> MAEGNTLISVDYEIFGKVQGVFFRKHTQAEGKKLGLVGWVQNTDRGTVQGQLQGPISKVRHMQEWLETRGSPKSHIDKANFNNEKVILKLDYSDFQIVK

Here we used a pair of thermophilic/mesophilic acylphosphatases homologues (acylphosphatase from hyperthermophilic archaeon Pyrococcus horikoshii (PhAcP) and human common-type acylphosphatase (HuAcP)) as a model to study how local flexibility of the active site affects the enzymatic activity. Despite remarkable conservation of sequence and structure at the active site, the catalytic activity of the thermophilic PhAcP is significantly poorer as compared with its mesophilic homologue HuAcP at low temperatures. The salt-bridge between the active-site residue Arg-20 and the C-terminal carboxyl group is found only in thermophilic PhAcP but not in mesophilic HuAcP. Taken together, our data suggest that the presence of the salt-bridge between the C-terminal carboxyl group and the active-site arginine residue increases the activation energy that results in a stronger temperature dependency of the enzymatic activity.

Importantly, the activation energy (52.5±2.5 kJmol−1) for HuG99 was analogous to that for PhWT (49.1±1.4 kJmol−1), while the activation energy for HuA99 (29.5±1.9 kJmol−1) and HuWT (37.6±3.1 kJmol−1) was comparable to that for PhG91A (32.1±1.7 kJmol−1). To provide further insights into how the active-site salt-bridge affected the enzymatic activity of acylphosphatases, we calculated and summarized the free energy (ΔG#), enthalpy (ΔH#), and entropy (ΔS#) of activation, as well as the changes of these parameters (ΔΔG#, ΔΔH#, ΔΔS#) upon the removal of the active-site salt-bridge. The values of ΔΔH# and TΔΔS# for HuWT were somewhat lower than those for HuA99.> MAWKDCIIQRYKDGDVNNIYTANRNEEITIEEYKVFV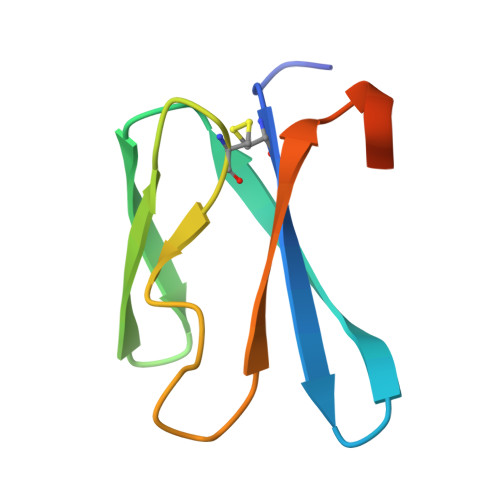NEACHPYPVILPDRSVLSGDFTSAYLEHHHHHH>[4x]MAHHHHHHMVNVAVIGAAGGIGQSLSLLLLRELPFGSTLSLYDVVGAPGVAADLSHIDRAGITVKHAAGKLPPVPRDPALTELAEGVDVFVIVAGVPRKPGMTRDDLFNVNAGIVMDLVLTCASVSPNACFCIVTNPVNSTTPIAAQTLRKIGVYNKNKLLGVSLLDGLRATRFINNARHPLVVPYVPVVGGHSDVTIVPLYSQIPGPLPDESTLKEIRKRVQVAGTEVVKAKAGRGSATLSMAEAGARFTMHVVKALMGLDTPMVYAYVDTDGEHECPFLAMPVVLGKNGIERRLPIGPITTVEKEMLEEAVGVVKKNIAKGETFARSKL;> MAHH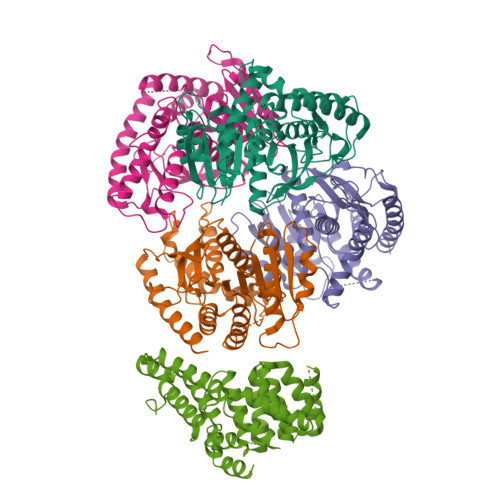HHHHMDCSTGAAIGQQFAKDAFHMHGGVGVGPTGNSEHDVLMNEMMMVQTPTGPAGEWTHQFAAYQGQQQQQQQQHPQELAMRHQQNDAFMLRQQQEMEEAFCTFCTTHPHSHAHSHQPQGLVGPAMMGPQIMPPMMFGPGTGGFMMGAPPMMPYASMKFAGDAAMAAANNTNMTQGATATSTTSVQQELQQQSSDNGWVEKLRDAEWAQDYSDAQVFTLEGQSEQTMEEHAKNSEFYQFMDKIRSKELLIDEETGQLVQGPGPDPDAPEDAEYLKEWAAAEGLNMPPGFFEHMMQRPQGNNEQAEGRLFDGSNDALMDDGALDNAADVEEWVREYAEAQEQLQRVQNETNYPFEPNNPYMYHDKPMEEGIAMLQLANMAEAALAFEAVCQKEPENVEAWRRLGTTQAENEKDCLAIIALNHARMLDPKDIAVHAALAVSHTNEHNVGAALQSLRSWLLSQPQYEHLGLVDLREVAADEGLDEVPEENYFFAAPSEYRDCCTLLYAAVEMNPNDPQLHASLGVLHNLSHRFDEAAKNFRRAVELRPDDAHMWNKLGATLANGNRPQEALEAYNRALDINPGYVRVMYNMAVSYSNMAQYPLAAKHITRAIALQAGGTNPQGEGSRIATRGLWDLLRMTLNLMDRSDLVEASWQQDLTPFLREFGLEEMAV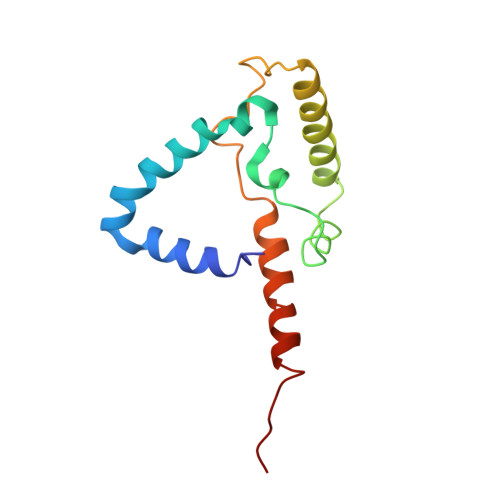> PQSFTSIARIGDYILKSPVLSKLCVPVANQFINLAGYKKLGLKFDDLIAEENPIMQTALRRLPEDESYARAYRIIRAHQTELTHHLLPRNEWIKAQEDVPYLLPYILEAEAAAKEKDELDNIEVSK> MAFRKENKIKNNFSKIRITLASPEEILENSFGEVLKPETINYRTYKPERDGLFCERIFGPVKDFECHCGKYKRIRYRGIVCDRCGVEVTEKKVRRERMGHIHLVVPVAHIWYFRSLPNKIGYLLGLPTKKLDAIIYYERYVVIQPGVAEGLSQLDLLSEEEYLDKLDEIERTHKGNQNLEDTNPDKFIAKIGAEAIYDLLCRVDLDSISYELRDRANTDGSQQRKTEALKRLQVVESFRASKGVNRPEWMVMKVIPVIPPDLRPLVPLDGGRFATSDLNDLYRRVIIRNNRLKRLIEIKAPEVILRNEKRMLQEAVDSLFDNSRKSSAVKSDNNRPLKSLSDSLKGKQGRFRQNLLGKRVDYSARSVIVVGPELKMHECGLPKDMAAELYKPFIIRKLIERGIVKTVKSAKKIVDRKEPVIWDILEYVMKGHPVLLNRAPTLHRLGIQAFQPKLIEGKAIQLHPLSCTAFNADFDGDQMAVHLPLSNEAILEAQLLMLASHNILNPANGAPITVPSQDMVLGLYYITKLRPNTKGHGLIFYGPEEATIAYNEGKVDIHAPIKVYVEDYENGELVRRMVETSVGRLMVNEYVPKKVGYVNEVLGKKALRDIIGSVIKICGVATTAKFLDDIKNLGYYMAFKGGLSFNLADVLIPDEKDQLIQEGYTAVEQIMQDYSMGFITFNERYNQIIDTWTH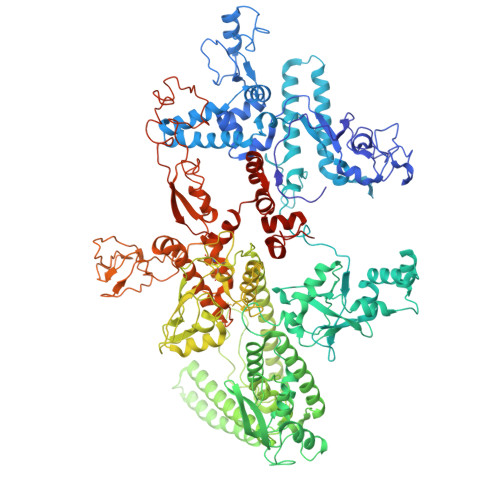INGRLSNVLIKQLSSDNDGFNSVFMMMDSGARGSKEQIRQLSGMRGLMAKPQKSGAEGGQIIENPILSNFKEGLSVLEYFISTHGARKGLADTALKTADAGYLTRRLVDVSHDVIITEEDCGTLRGLLTTELKQNEDVVASLYERILGRVSVHDIIHPTTGDIIVRAGEEIREQAAQIIEDSPIEAVEIRSVLTCESKKGVCAKCYGRNLATNRMVQRGEVVGVIAAQSIGEPGTQLTLRTFHVGGIASNVATENSLLSKYDGILEFEELRAVDATDESHQVVVSRMTELRIADPNTGIILANHNIPYGAKLFFRQGDAVKKGDKIIEWDPFNAVIVSEVAGTLSFEGVVENVTFKMESDETTGLKEKIIIESKDKTMAPYARIIDENGEMLKNYSLPMGAHVVKDDGDTVKVGEILVKIPRSVGKAGDITGGLPRVTELFEARNPSNPAIVSEIDGEIGFGKLKRGNREITVTSKLGEEKKYLIPLSKQLLVQENDFVRAGTPLSDGAITPADILAIKGPTAVQEYIVNEVQDVYRLQGVKINDKHFEVIVRQMMRKVEIVDPGDTLFLEQQVVDKFEVMEENDRIWGKKVVIDAGDSQVLKAGQIVTARKLRDENSMLKRKDLKIVKVRDAKSATASQILQGITRAALQTKSFMSAASFQETTKVLNEAAICGKTDYLEGLKENVICGHLIPAGTGLRDYEKLVVMHRDDYEKATAERKSFLSEPTAEPAMEEAPSEHHHHHH> RDFNNLTKGLCTINSWHIYGKDNAVRIGEDSDVLVTRGPYVSCDPDECRFYALSQGTTIRGKHSNGTIHDRSQYRALISWPLSSPPTVYNSRVECIGWSSTSCHDGKTRMSICISGPNNNASAVIWYNRRPVTEINTWARNILRTQESECVCHNGVCPVVFTDGSATGPAETRIYYFKE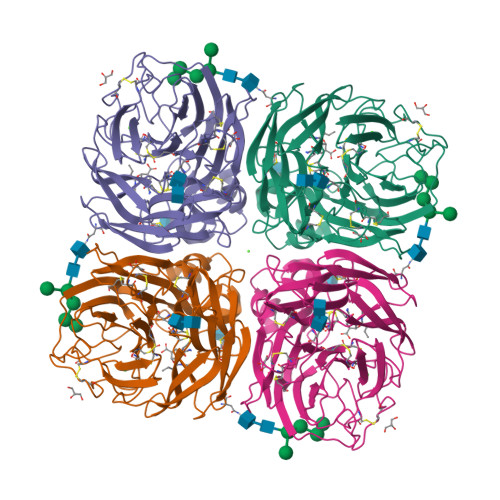GKILKWEPLAGTAKHIEECSCYGERAEITCTCRDNWQGSNRPVIRIDPVAMTHTSQYICSPVLTDNPRPNDPTVGKCNDPYPGNNNNGVKGFSYLDGVNTWLGRTISIASRSGYEMLKVPNALTDDKSKPTQGQTIVLNTDWSGYSGSFMDYWAEGECYRACFYVELIRGRPKEDKVWWTSNSIVSMCSSTEFLGQWDWPDGAKIEYFL> GSHMASPNGQTKPLPALKLALEYIVPAMNKHGICVVDDFLGKETGQQIGDEVRALHDTGKFTDGQLVSQKSDSSKDIRGDKITWIEGKEPGCETIGLLMSSMDDLIRHCNGKLGSYKINGRTKAMVACYPGNGTGYVRHVDNPNGDGRCVTCIYYLNKDWDAKVSGGILRIFPEGKAQFADIEPKFDRLLFFWSDRRNPHEVQPAYATRYAITVWYFDADERAAAKVKYLTGE;> XYVWLTDTWVLSRT

The degradation of HIFα subunits is promoted by post-translational hydroxylation of prolyl-residues located in its N/C-terminal oxygen dependent degradation domains (NODD and CODD). These dioxygen-sensitive reactions are catalysed by 2-oxoglutarate (2OG) and Fe(II) dependent prolyl hydroxylases (PHD 1–3 in humans). The human PHDs catalyse hydroxylation of prolyl-residues within the N/C terminal ODDs of HIF-1/2/3α and are negative regulators of the transcriptionally regulated hypoxic response.

We successfully crystallized cPHD2 in the presence of a 14-residue NCCP (3C), obtained in a RaPID with five rounds of screening. Multiple crystals were obtained in the presence of 3C and active site binding inhibitors, such as NOG (N-oxalylglycine, a close 2OG analogue) and FG2216, in the hexagonal P65 crystal form. Consistent with the reported NMR studies, we obtained multiple crystal structures revealing that 3C binds in the region of cPHD2 immediately to the N-terminal side of the core distorted double stranded β-helix (DSBH) fold of PHD2. Interestingly, within the crystal lattice, 3C ‘slots’ into a tight groove between the non-DSBH β1 of one cPHD2 molecule and the C-terminal α4 (that is also involved in the P63 crystal packing) of a neighbouring symmetry related cPHD2 molecule. Binding of 3C at the interface of two symmetry related PHD2 monomers likely promotes contacts productive for crystallization in part via projecting part of the C-terminal helix α4 (aa 400–404) away from the active site, in a manner that maintains interactions with substrates that are required for catalysis. In the cPHD2.3C complex structures, 3C adopts a rectangular fold comprising two (almost) planar distorted β-strands connected by two type II beta turns with DY1, D6, W8 and T13 at its four corners; most of the side chains do not protrude extensively. 3C forms extensive backbone-to-backbone interactions with cPHD2 β1 (aa 204–214) and three residues located at the N-terminus (187–189) within the same cPHD2 monomer and six residues (399–404) located at the C-terminus of a symmetry related cPHD2 molecule. In addition, there are backbone to side-chain polar interactions between L188PHD2 and F213PHD2 with R123C, and A399PHD2 with T53C, as well as side-chain to side-chain electrostatic/H-bond interactions of D212PHD2 with T133C and S113C, and of K186PHD2 with YD13C. Although the 3C interacting PHD2 residues are well-conserved in all three human PHDs, they are different in other 2OG-oxygenases including the ribosomal prolyl hydroxylase (OGFOD1, Z = 17.4), nucleic acid demethylases (e.g., FTO, Z = 14.4), phytanoyl-CoA dioxygenase (PAHX, Z = 13.3)38 and factor inhibiting HIF (FIH, Z = 10.8), providing a structural basis for the high selectivity of 3C and related NCCPs for the PHDs.>MDLRDIDLNLLVVFNQLLLDRSVSTAGEKLGLTQPAVSNSLKRLRTALNDDLFLRTSKGMEPTPYALHLAEPVIYALNTLQTALTTRDSFDPFASTRTFNLAMTDIGEMYFMPPLMEALAQRAPHIQISTLRPNAGNLKEDMESGAVDLALGLLPELQTGFFQRRLFRTRYVCMFRKDHPSAKSPMSLKQFSELEHVGVVALNTGHGEVDGLLERAGIKRRMRLVVPHFIAIGPILHSTDLIATVPQRFAVRCEVPFGLTTSPHPAKLPDIAINLFWHAK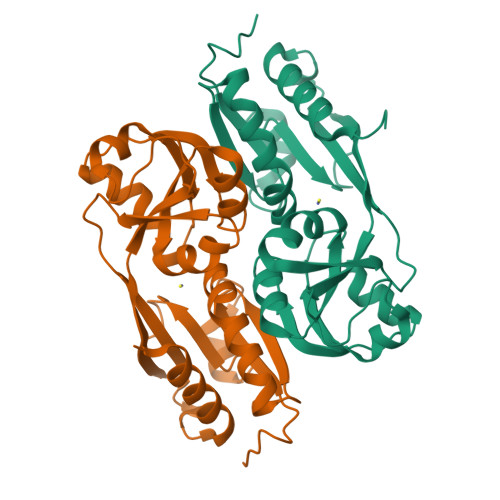YNRDPGNMWLRQLFVELFSEARHHHHHH[2x]>[2x]MQPDMS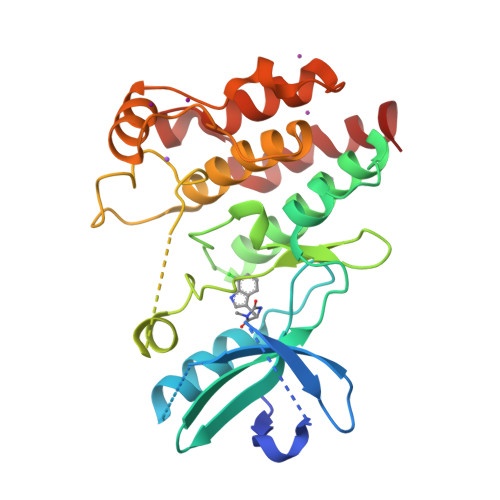LNVIKMKSSDFLESAELDSGGFGKVSLAFHRTQGLMIMKTVYKGPNCIEHNEALLEEAKMMNRLRHSRVVKLLGVIIEEGKYSLVMEYMEKGNLMHVLKAEMSTPLSVKGRIILEIIEGMAYLHGKGVIHKDLKPENILVDNDFHIKIADLGLASFKMWSKLNNEEHNELREVDGTAKKNGGTLYYMAPEHLNDVNAKPTEKSDVYSFAVVLWAIFANKEPYENAIAEQQLIMAIKSGNRPDVDDITEYCPREIISLMKLCWEANPEARPTFPGIEEKFRPFYLSQLE>VLDSFEILKALKSLDLLKNAPAWWWPNALKFEALLGAVLTQNTKFEAVLKSLENLKNAFILENDDEINLKKIAYIEFSKLAECVRPSGFYNQKAKRLIDLSGNILKDFQSFENFKQEVTREWLLDQKGIGKE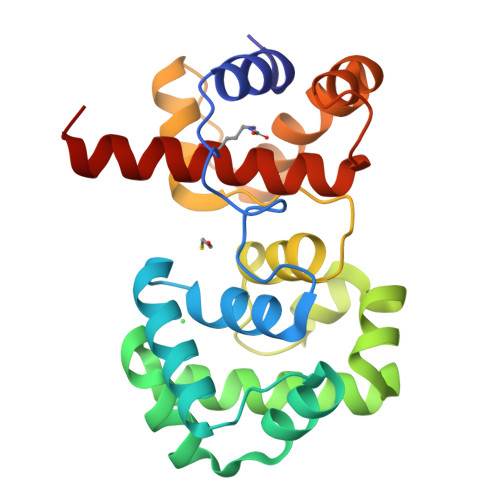SADAILCYACAKEVMVVDKYSYLFLKKLGIEIEDYDELQHFFEKGVQENLNSALALYENTISLAQLYARFHGKIVEFSKQKLELKL[2x]> GGGTMQVQCQQSPVLAGSATLVALGALALYVAKPSGYGKHTESLKPAATRLPARAAWFLQELPSFAVPAGILARQPLSLFGPPGTVLLGLFCVHYFHRTFVYSLLNRGRPYPAILILRGTAFCTGNGVLQGYYLIYCAEYPDGWYTDIRFSLGVFLFILGMGINIHSDYILRQLRKPGEISYRIPQGGLFTYVSGANFLGEIIEWIGYALATWSLPALAFAFFSLCFLGLRAFHHHRFYLKMFEDYPKSRKALIPFIF

SRD5α2 is highly expressed in male reproductive systems to convert testosterone to 5α-dihydrotestosterone (DHT), the major steroid hormone for androgen receptor. SRD5αs belong to a large group of eukaryotic membrane-embedded steroid reductases, which also include sterol reductases such as the 7-dehydrocholesterol reductase (DHCR7) that catalyzes the last step in cholesterol biosynthesis in humans. Although these steroid/sterol reductases share very little sequence similarity, they all use NADPH as the cofactor to reduce specific carbon-carbon double bonds in their steroid substrates. To our knowledge, the reported structure of human SRD5α2 with the dualsteric ligand NADP-DHF represents the first structure of eukaryotic membrane-embedded steroid reductase.

Human SRD5α2 was expressed in insect Sf9 cells and purified in the presence of finasteride and crystallized in lipidic mesophase with a space group of P622. The structure was determined to 2.8-Å resolution by molecular replacement based on a structural model from de novo prediction since we failed to use anomalous diffraction data to solve the structure. Unlike the bacterial sterol reductase MaSR121, the structure of SRD5α2 contains 7 TMs (TM1-7) connected by 6 loops (L1-6). In addition, the N-terminal residue C5N (superscripts indicate location of the residues hereafter) forms a disulfide bond with C133L4 in loop 4 (L4), suggesting an ER luminal location of the N-terminal side because of the reducing environment of the cytosol. The structure of SRD5α2 revealed a large cavity inside the 7-TM domain at the cytosolic side formed by all 7 TMs and L1, L3 and L5. The cavity is completely occluded from the cytosol with only one opening on the side of 7-TM domain between TM1 and TM4. Strikingly, after ligand fitting, the distance between the nicotinamide C-4 atom of NADPH and the C-2 atom of finasteride is shorter than 2Å, suggesting the formation of a covalent bond. The same study indicated that SRD5α2 could catalyze the hydride transfer from NADPH to finasteride, leading to the formation of a covalent bond between the nicotinamide C-4 atom of NADPH and the C-2 atom of finasteride17, highly consistent with our structural observation. It is likely that SRD5α2 took endogenous NADPH during recombinant protein expression to catalyze the reaction with finasteride supplemented in protein buffers to generate the NADP-DHF intermediate, which was stable enough to be captured in our SRD5α2 crystals. In contrast to the highly polar environment for NADP, the binding pocket of DHF is largely hydrophobic, where the core ring structure of DHF interacts with hydrophobic residues from TMs 1, 2, 4 and 7. In our structure, both the C-3 carbonyl and the N-4 amine groups of DHF form hydrogen bonds with E57TM2.>MTPHINAKIGDFYPQCLLCGDPLRVSYIAKKFLQDAKEITNVRNMLGFSGKYKGRGISLMGHGMGIASCTIYVTELIKTYQVKELLRIGTCGAISPKVGLKDIIMATGASTDSKTNRVRFLNHDLSATPDFELSLRAYQTAKRLGIDLKVGNVFSSDFFYSFETHAFDLMAKYNHLAIEMEAAGLYATAMELNAKALCLCSVSDHLITKEALSP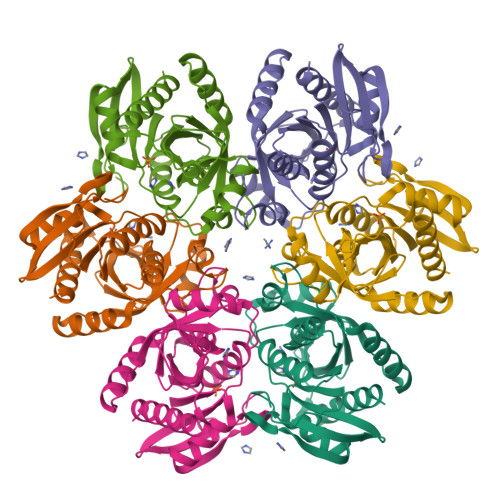KERVESFDNMIILALEMMS[6x]>THSLHNAAPREALTDTIMAAKIRHNLTFEALAQGTGLSLAFVTAALLGQHALPEPAARTVAAKLGLDEEAVLLLQTIPLRGSIPGGVPTDPTIYRFYEMLQVYGSTLKALVHEQ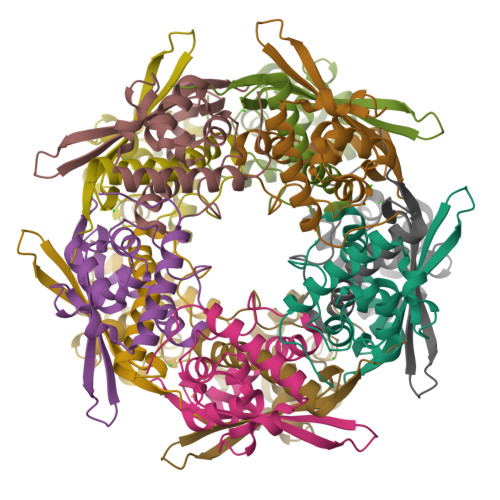FGDGIISAINFKLDIKKVADPDGGERAVITLDGKYLPTKPF[20x]>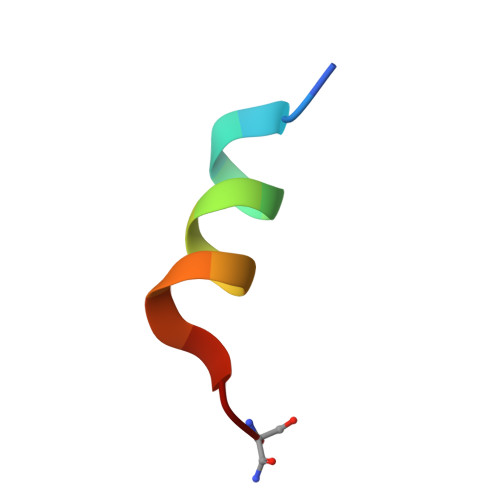 KETAAAKAERQHMDS>[3x]MSLKKVVIIGGGAAGMSAASRVKRLKPEWDVKVFEATEWVSHAPCGIPYVVEGLSTPDKLMYYPPEVFIKKRGIDLHLNAEVIEVDTGYVRVRENGGEKSYEWDYLVFANGASPQVPAIEGVNLKGVFTADLPPDALAIREYMEKYKVENVVIIGGGYIGIEMAEAFAAQGKN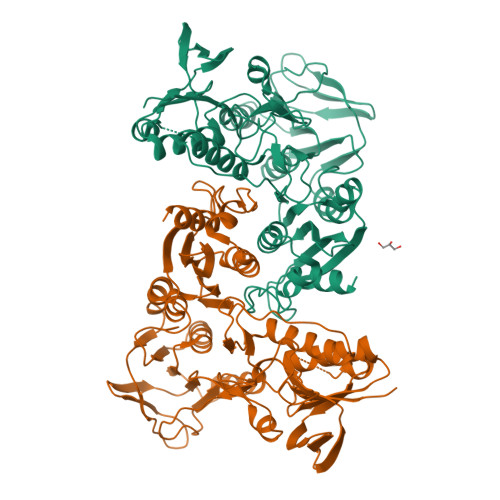VTMIVRGERVLRRSFDKEVTDILEEKLKKHVNLRLQEITMKIEGEERVEKVVTDAGEYKAELVILATGIKPNIELAKQLGVRIGETGAIWTNEKMQTSVENVYAAGDVAETRHVITGRRVWVPLAPAGNKMGYVAGSNIAGKELHFPGVLGTAVTKFMDVEIGKTGLTEMEALKEGYDVRTAFIKASTRPHYYPGGREIWLKGVVDNETNRLLGVQVVGSDILPRIDTAAAMLMAGFTTKDAFFTDLAYAPPFAPVWDPLIVLARVLKEGHHHHHH>[22x]MAQVINTNSLS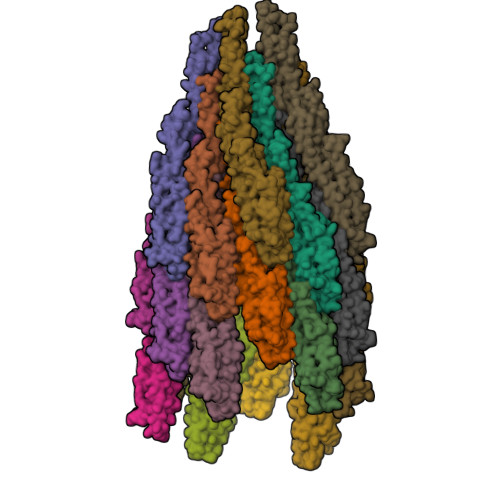LITQNNINKNQSALSSSIERLSSGLRINSAKDDAAGQAIANRFTSNIKGLTQAARNANDGISVAQTTEGALSEINNNLQRIRELTVQASTGTNSDSDLDSIQDEIKSRLDEIDRVSGQTQFNGVNVLAKDGSMKIQVGANDGQTITIDLKKIDSDTLGLNGFNVNGKGETANTAATLKDMSGFTAAAAPGGTVGVTQYTDKSAVASSVDILNAVAGADGNKVTTSADVGFGTPAAAVTYTYNKDTNSYSAASDDISSANLAAFLNPQARDTTKATVTIGGKDQDVNIDKSGNLTAADDGAVLYMDATGNLTKNNAGGDTQATLAKVATATGAKAATIQTDKGTFTSDGTAFDGASMSIDANTFANAVKNDTYTATVGAKTYSVTTGSAAADTAYMSNGVLSDTPPTYYAQADGSITTTEDAAAGKLVYKGSDGKLTTDTTSKAESTSDPLAALDDAISQIDKFRSSLGAVQNRLDSAVTNLNNTTTNLSEAQSRIQDADYATEVSNMSKAQIIQQAGNSVLAKANQVPQQVLSLLQG>[2x]MSVFVSGANGFIAQHIVDLLLKEDYKVIGSARSQEKAENLTEAFGNNPKFSMEVVPDISKLDAFDHVFQKHGKDIKIVLHTASPFCFDITDSERDLLIPAVNGVKGILHSI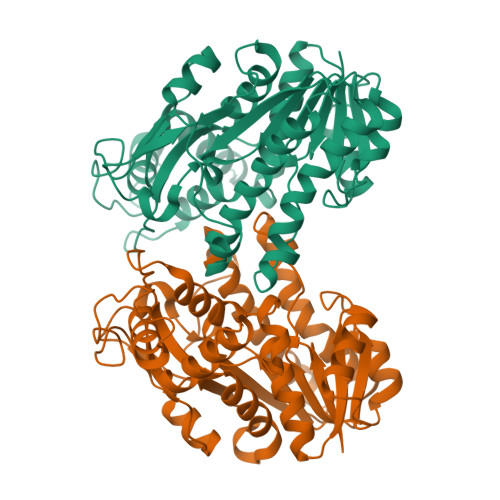KKYAADSVERVVLTSSYAAVFDMAKENDKSLTFNEESWNPATWESCQSDPVNAYCGSKKFAEKAAWEFLEENRDSVKFELTAVNPVYVFGPQMFDKDVKKHLNTSCELVNSLMHLSPEDKIPELFGGYIDVRDVAKAHLVAFQKRETIGQRLIVSEARFTMQDVLDILNEDFPVLKGNIPVGKPGSGATHNTLGATLDNKKSKKLLGFKFRNLKETIDDTASQILKFEGRI>MQKITVPTWAEINLDNLRFNLNNIKNLLEEDIKICGVIKADAYGHGAVEVAKLLEKEKVDYLAVARTAEGIELRQNGITLPILNLGYTPDEAFEDSIKNKITMTVYSLETAQKINEIAKSLGEKACVHVKIDSGMTRIGFQPNEESVQEIIELNKLEYIDLEGMFTHFATADEVSKEYTYKQANNYKFMSDKLDEAGVKIAIKHVSNSAAIMDCPDLRLNMVRAGIILYGHYPSDDVFKDRLELRPAMKLKSKIGHIKQVEPGVGISYGLKYTTTGKETIATVPIGYADGFTRIQKNPKVLIKGEVFDVVGRICMDQIMVRIDKDIDIKVGDEVILFGEGEVTAERIAKDLGTINYEVLCMISRRVDRVYMENNELVQINSYLLK[4x]

Alanine racemase (Alr) is a pyridoxal-5′-phosphate (PLP)-dependent enzyme that catalyzes the reversible racemization of l- and d-alanine. Since d-alanine is an essential component of the bacterial cell-wall peptidoglycan, and there are no known Alr homologs in humans, this enzyme is being tested as an antibiotic target. Three crystal structures of C. difficile Alr (CdAlr), corresponding to the complex with PLP, the complex with cycloserine and a K271T mutant form of the enzyme with bound PLP, are presented. The structures are prototypical Alr homodimers with two active sites in which the cofactor PLP and cycloserine are localized.

The first is the structure of the enzyme in complex with the PLP cofactor (CdAlrPLP). Uniquely, the CdAlrPLP crystal structure is a tetramer, while the other two structures are dimers. The CdAlrPLP structure gives the highest resolution data, but it also has the highest level of disorder and lacks several residues in proximity to the binding cavity and the dimer interface. Key disordered regions in monomer A include all residues from Lys258 to Thr279; in monomer B the disordered residues are Ser133–Gly139 and Glu173–Glu177, while in monomer D residues Gly197–Ile200 are disordered. The CdAlrPLP tetramer is a dimer of two almost identical dimers, with an r.m.s.d. of 0.274 Å for the superpositioning of main-chain atoms of the dimers. Each dimer is structurally similar to the homodimers of CdAlrK271T (r.m.s.d. of 0.288 Å to one dimer and 0.361 Å to the other) and CdAlrcycloserine (r.m.s.d. of 0.397 Å to one dimer and 0.511 Å to the other). Subsequent peptide sequencing revealed that the minor species corresponded to amino acids 1–271 and 272–382 and that the two peptides resulted from a cleavage of unknown nature at position 271.5-(2-methylphenyl)thiophene-2-carboxylic acid | C12 H10 O2 S | 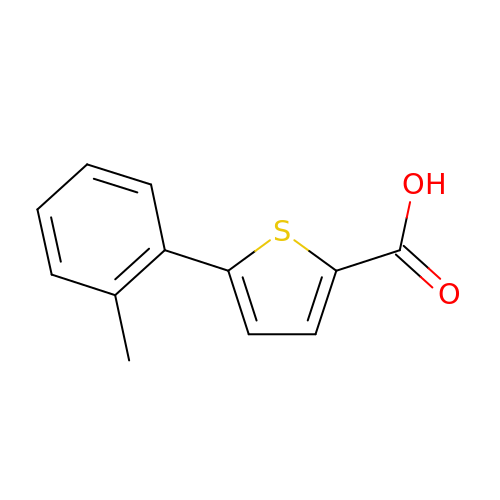BSOIGQKKGJNDJD-UHFFFAOYSA-N>GGDPHMMFGKKKNNGGSSTARYSAGNKYNTLSNNYALSAQQLLNASKIDDIDSMMGFERYVPPQYNGRFDAKDIDQIPGRVGWLTNMHATLVSQETLSSGSNGGGNSNDGERVTTNQGISGVDFYFLDEEGGSFKSTVVYDPYFFIACNDESRVNDVEELVKKYLESCLKSLQIIRKEDLTMDNHLLGLQKTLIKLSFVNSNQLFEARKLLRPILQDNANNNVQRNIYNVAANGSEKVDAKHLIEDIREYDVPYHVRVSIDKDIRVGKWYKVTQQGFIEDTRKIAFADPVVMAFDIETTKPPLKFRDSAVDQIMMISYMIDGEGFLITNREIISEDIEDFEYTPKPEYPGFFTIFNENDEVALLQRFFEHIRDVRPTVISTFNGDFFDWPFIHNRSKIHGLDMFDEIGFAPDAEGEYKSSYCSHMDCFRWVKRDSYLPQGSQGLKAVTQSKLGYNPIELDPELMTPYAFEKPQHLSEYSVSDAVATYYLYMKYVHPFIFSLCTIIPLNPDETLRKGTGTLCEMLLMVQAYQHNILLPNKHTDPIERFYDGHLLESETYVGGHVESLEAGVFRSDLKNEFKIDPSAIDELLQELPEALKFSVEVENKSSVDKVTNFEEIKNQITQKLLELKENNIRNELPLIYHVDVASMYPNIMTTNRLQPDSIKAERDCASCDFNRPGKTCARKLKWAWRGEFFPSKMDEYNMIKRALQNETFPNKNKFSKKKVLTFDELSYADQVIHIKKRLTEYSRKVYHRVKVSEIVEREAIVCQRENPFYVDTVKSFRDRRYEFKGLAKTWKGNLSKIDPSDKHARDEAKKMIVLYDSLQLAHKVILNSFYGYVMRKGSRWYSMEMAGITCLTGATIIQMARALVERVGRPLELDTDGIWCILPKSFPETYFFTLENGKKLYLSYPCSMLNYRVHQKFTNHQYQELKDPLNYIYETHSENTIFFEVDGPYKAMILPSSKEEGKGIKKRYAVFNEDGSLAELKGFELKRRGELQLIKNFQSDIFKVFLEGDTLEGCYSAVASVCNRWLDVLDSHGLMLEDEDLVSLICENRSMSKTLKEYEGQKSTSITTARRLGDFLGEDMVKDKGLQCKYIISSKPFNAPVTERAIPVAIFSADIPIKRSFLRRWTLDPSLEDLDIRTIIDWGYYRERLGSAIQK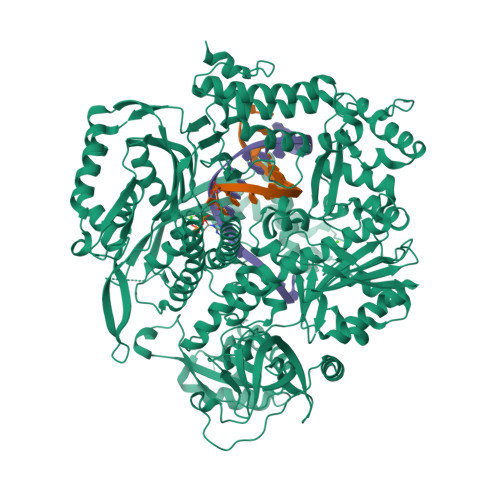IITIPAALQGVSNPVPRVEHPDWLKRKIA[2x]> LAAALEGPYPVEEIRLPRAGGPLGLSIVGGSDHSSHPFGVQEPGVFISKVLPRGLAARSGLRVGDRILAVNGQDVRDATHQEAVSALLRPCLELSLLVRRDPAPPGLRELCIQKAPGERLGISIRGGARGHAGNPRDPTDEGI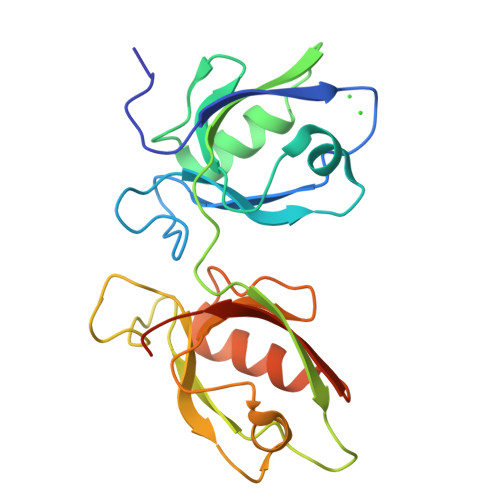FISKVSPTGAAGRDGRLRVGLRLLEVNQQSLLGLTHGEAVQLLRSVGDTLTVLVCDGFEASTDAALEVS>GSHMRQPIALISVHGDPAADVGHESAGGQNIYVRQLGEALAAAGWHVDMFTRKTDPNDPDVIEHSPHCRTIRLQAGPLTYIPREKLFETLPKFVEAFKAYHAKYGYPLIHTNYWLSGWVGWQLRQQFNFQWLHTYHSLGVVKYQVASEQAQRDETRLMVEKAILENADCVIVTSPQ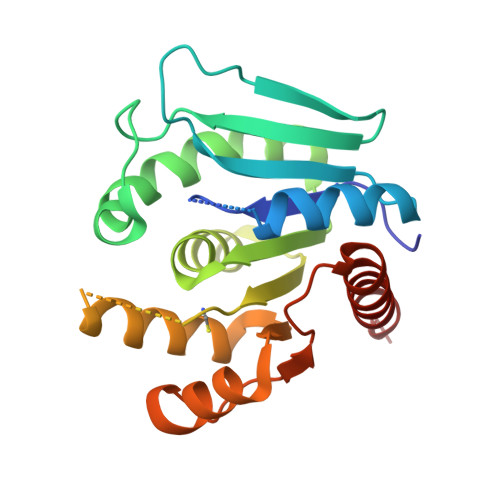EEAYLRRWVSKAGQTRLIPCGTNWEAIALQMGQLYRQLFAASL[4x]Here we analyzed the endogenous regulation of anthraquinone (AQ) pigments, which give Photorhabdus species their characteristic orange-to-red coloration during exponential growth. , AQs are aromatic polyketides produced by a type II polyketide synthase system (PKS), which is rarely found in Gram-negative bacteria. After partial cyclization, the AntF-bound intermediate is further processed to a heptaketide by the unusual chain length shortening lyase AntI. , Spontaneous oxidation of precursor compounds results in the red pigment AQ-256, which exhibits a tricyclic structure. Metabolic and proteomic analyses following CA treatment show that CA inhibits AntI, a key enzyme in the final step of AQ-256 biosynthesis.

The crystal structure of AntI in complex with CA reveals that cinnamic acid functions as a competitive inhibitor by inducing specific structural rearrangements in the lyase, resulting in noncovalent, reversible inhibition. The complex forms a homodimer with a single subunit in the asymmetric unit, and CA is well-defined in the Fo-Fc electron density map and occupies the substrate binding channel. In the open state, the Pro281-Arg283 loop (region I) and Tyr20 are exposed to solvent. However, upon CA binding, this segment undergoes a 90° rotation, causing the side chain of Arg282 to flip inward, while Tyr20 rotates by 120°. These structural rearrangements facilitate π-stacking between Arg282 and Tyr20, leading to the formation of two strong salt bridges between Arg282 and Asp327. In the AntI:CA complex, the catalytic triad remains perfectly aligned (region II), with the active site nucleophile Ser245 positioned just 3.4 Å from the styrene moiety of CA. However, the conjugated π-electron system of the aromatic ring stabilizes the double bond, preventing Ser245 from forming a covalent bond with the ligand. The styrene residue of CA engages in cation-π stacking with Arg24 and π-π stacking with Phe27, while its carboxylate group forms hydrogen bonds with the backbone amides of Gly173, Leu174, and Asp175. However, in the CA-bound structure, the carboxylate group of CA displaces Gly173 and induces a 37° rotation of its carbonyl group. This structural rearrangement imposes geometric constraints that generate energetically unfavorable φ- and ψ-dihedral angles in the protein backbone within region II, counteracting the otherwise favorable ligand interactions at the active site.

> GSSHHHHHHSGDPASMNNKNKPNRISPELLATCGYFMPRIFFLNSQYAPQVHWGDVVAALSHFPAGNLDLSSEEFWYEWMINWSKVGDSYINIANSAKSEVSHVRALRSAAACYHWAEFMYFSDRSRKIQLREYIRSCFLSSIKYSDLLVDHQYIVVDKFHMPFFLIFPKGYKEEENHPLPCVILSNGLDSMTEIEILSLAEFFLGKNMAVAIFDGPGQGINLGKSPIAIDMELYVSSIVKLLEDDARINSNLLCFLGISFGGYFALRVAQRIGDKFCCIVNLSGGPEIAEFDKLPRRLKEDFQFAFMQDNSHMQSIFDEIKLDISLPCKTKVFTVHGELDDIFQIDKVKKLDQLWGDNHQLLCYESEAHVCLNKINEYMIQVSDWVSEQFWLNGYKKG6-PHOSPHOCYCLOPHELLITOL | C7 H15 O9 P | 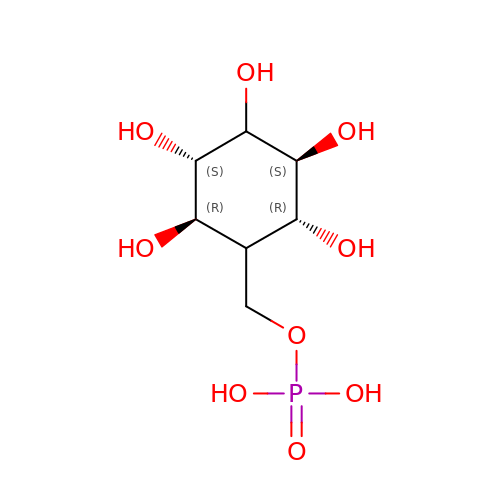UJSILGAUEGUBGA-NYLBLOMBSA-N>MGTFTLHQGQTNLIKSFFRNYYLNAELELPKDMELREFALQPFGSDTYVRHLSFSSSEELRDYLVNRNLPLHLFYSSARYQLPSARNMEEKAWMGSDLLFDIDADHLCKLRSIRFCPVCGNAVVSEKCERDNVETLEYVEMTSECIKRGLEQTRNLVEILEDDFGLKPKVYFSGNRGFHVQVDCYGNCALLDSDERKEIAEYVMGIGVPGYPGGSENAPGWVGRKNRGINGVTIDEQVTIDVKRLIRIPNSLHGKSGLIVKRVPNLDDFEFNETLSPFTGYTIFLPYITIETEVLGSIIKLNRGIPIKIKSSIGIYLHLRNLGEVKAYVR[2x];>MALDVKKYPFIKSLDDELKKYGGGITLTDLLLNSTTLIDQAKDRIQKTKSGDELPHYVSYNEPVLVFYTTLLSLAILNDVKLIRRYAYAEAKQFRSLLHTENEENLLEISKLLDLKINR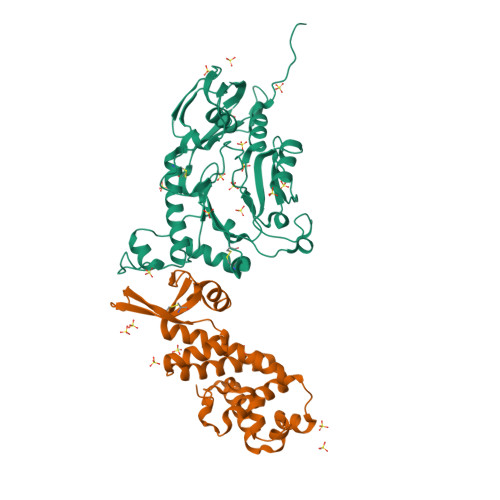CDPIKFYLEKKRRIIQKEFCVHFIDYLKYTKDLKEDWKLSGQILHKGYVYLDKNQLIGLIAESIKSKIVEMIRPLNLKEIPEKLKSLIERRGI[2x]>[2x]MGGGFAQDKNPLSTFGPDLNEFSRDVNFLTLAKNSDFIYLRASGSGTGKLRIDNKFLEFAKECRRLGI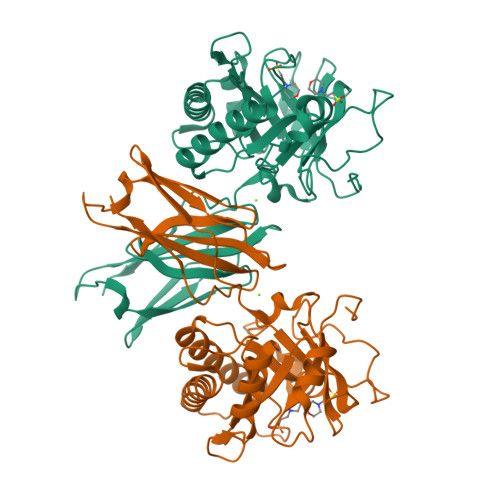PCGAYHFAKPSKDLDSAVIQADQFIDVLQQGFGDGDYGDLFPVLDVETPTDKSLTTTELVNWIDRFRDRFEEKTRRRLMLYTGLFFIGLYDDFKVPGKGYPLSDMPLWIAMYTRIPSNPRIPPNVGGWKRWTMWQFTDEGKLDGVGSPVDLNWGPNSIDSLMPPSAVTGLNAYISGNKIFVNWTANKEDDLNGYNVFVNDNYAGTLPRKATKIVIDKSRFYLPKGKPIKISIEAFDITGDFSKERTEYILDNNGEFLGENLYFQ> IVGGRDCAEGECPWQALLVNEENEGFCGGTILNEFYVLTAAHCLHQAKRFTVRVGDRNTEQEEGNEMAHEVEMTVKHSRFVKETYDFDIAVLRLKTPIRFRRNVAPACLPEKDWAEATLMTQKTGIVSGFGRTHEKGRLSSTLKMLEVPYVDRSTCKLSSSFTITPNMFCAGYDTQPEDAC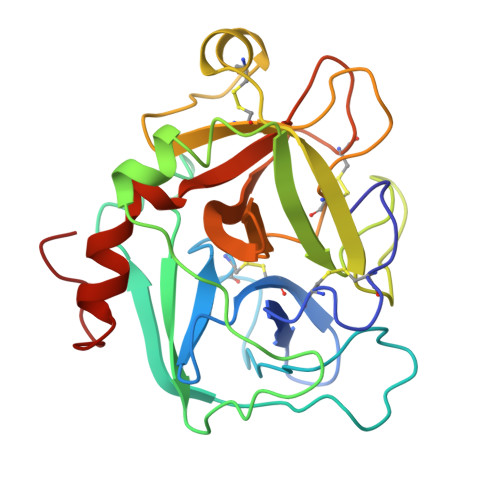QGDSGGPHVTRFKDTYFVTGIVSWGEGCARKGKFGVYTKVSNFLKWIDKIMKARAGAAGS> GPGHMAQVAGAALSQAGWYLSDEGIEACTSSPDKVNVNDIILIALNTDLRTIGKKFLPSDINSGKVE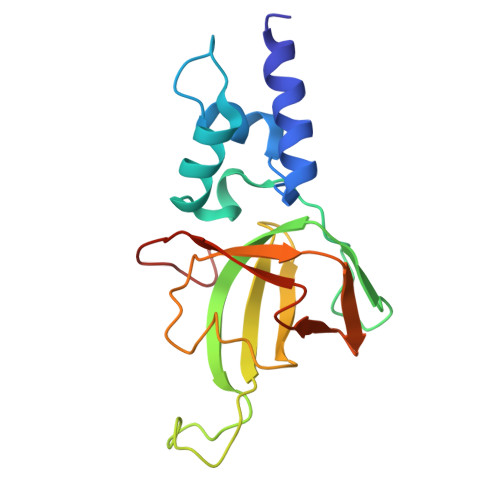KLEGPCVLQIQKIRNVAAPKDNEESQAAPRMLRLQMTDGHISCTAVEFSYMSKISLNTPPGTKVKLSGIVDIKNGFLLLNDSNTTVLGGEVEHLIEKW Here, we demonstrate that one such protease toxin from Escherichia coli, Cpe1, disrupts DNA replication and chromosome segregation by cleaving conserved sequences within the ATPase domain of type II DNA topoisomerases GyrB and ParE. Cpe1 belongs to the papain-like cysteine protease family and is associated with toxin delivery pathways, including the type VI secretion system and contact-dependent growth inhibition. The defining feature of this protease family is a conserved catalytic triad, consisting of a cysteine (Cys) thiol group, a histidine (His) imidazolium ring, and a third residue—either aspartate (Asp) or asparagine (Asn)—that orients and activates the imidazolium ring for peptide bond hydrolysis. Therefore, bacteria encode specific immunity proteins adjacent to their cognate toxin genes to prevent self-intoxication or harm to kin cells.

To circumvent this limitation, we co-purified Cpe1tox with its cognate immunity protein, Cpi1, which allowed us to obtain well-diffracting crystals. Using selenomethionine-substituted protein, we determined the crystal structure of the Cpe1tox–Cpi1 complex at a resolution of 1.87 Å. In our crystal structure, Cpe1 features a six-stranded antiparallel β-sheet flanked by five α-helices on either side, forming the typical α/β core that is characteristic of the PLCP family. The catalytic triad—Cys, His, Asp—is clearly evident and aligns with prior functional predictions. Despite sharing limited sequence identity with ABC transporter-associated proteases, a structural homology search using the DALI server identified ComA (Z-score = 16.3; RMSD of 1.9 Å across 121 aligned Cα atoms) and LahT (Z-score = 15.9; RMSD of 1.8 Å across 117 aligned Cα atoms) as the closest homologs. Interestingly, although Cpi1 binds to Cpe1 and they share a large interface (1,050 Å2), our crystal structure reveals that Cpi1 does not sterically occlude the active site of Cpe1. Instead, Cpi1 primarily interacts with a shallow hydrophobic concave region on the surface of Cpe1 that is located adjacent to the catalytic pocket. This binding region consists of a cluster of non-polar residues—L387, M390, A408, M426, W428, and V434—the hydrophobic properties of which are conserved across many T6SS- and CDI-associated Cpe1 toxins. We did not identify any enzymatic domain in or significant structural homologs of Cpi1, suggesting that its neutralization mechanism depends on binding to the hydrophobic concave region of Cpe1 rather than occlusion of its active site. However, when we mutated all four residues (Cpi1mut4), the resulting mutant lacked the ability to neutralize Cpe1 toxicity and failed to bind Cpe1 in vitro, despite being expressed at levels comparable to that of wild-type protein.

>MGSSHHHHHHSQDPAGGNWTVFDEVLDSNVIKQLTLTGCGAACGEMLLRDRYIFVTQNVIGTELTSMTSLANKLNKFDVGWEGNAVSESSLYALSNTGSWGAMMWDSGSKVGHWVLVKGVDDAGNVIIYDPYQGSRYLMTEQEFKEVWNGHSVYKP[2x];>[2x]MGIVFTNHNIDLLSVEFDEITKNCNYTFSVDGETAIFTARISIIRNIKGIKYSEELDKFIMSIMPLQPKVSKILGGVTWDCICGKEVGFPVRLIGK> LMKLYSLSVFYKGEPKAVLLKAAYDVSSFSFFQRSSVQEFMTFTSQLIVERSAKGSRASVKEQEYLCHVYV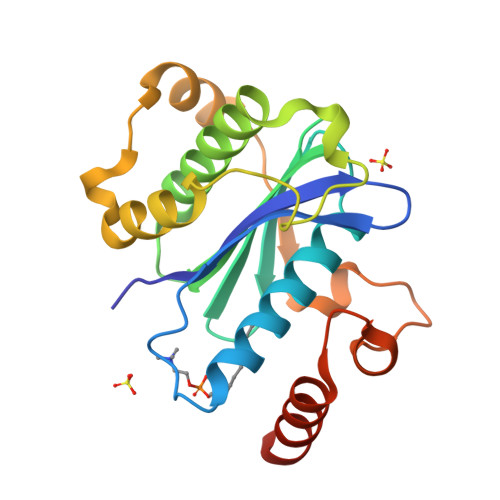RSDSLAGVVIADSEYPSRVAFTLLEKVLDEFSKQVDRIDWPVGSPATIHYTALDGHLSRYQNPREADPMSKVQAELDETKIILHNTMESLLERGEKLDDLVSKSEVLGTQSKAFYKTARKQNSCCAIM>MGFLVMIREVSMAKAIRVVLLCVSVLWVVPKECACRSNFSRNSSSSSSSSLRPLRQRPSSVNVGALFTYDSFIGRAAKPAVKAAMDDVNADQSVLKGIKLNIIFQDSNCSGFIGTMGALQLMENKVVAAIGPQSSGIAHMISYVANELHVPLLSFGATDPTLSSLQFPYFLRTTQNDYFQMHAIADFLSYSGWRQVIAIFVDDECGRNGISVLGDVLAKKRSRISYKAAITPGADSSSIRDLLVSVNLMESRVFVVHVNPDSGLNVFSVAKSLGMMASGYVWIATDWLPTAMDSMEHVDSDTMDLLQGVVAFRHYTIESSVKRQFMARWKNLRPNDGFNSYAMYAYDSVWLVARALDVFFRENNNITFSNDPNLHKTNGSTIQLSALSVFNEGEKFMKIILGMNHTGVTGPIQFDSDRNRVNPAYEVLNLEGTAPRTVGYWSNHSGLSVVHPETLYSRPPNTSTANQRLKGIIYPGEVTKPPRGWVFPNNGKPLRIGVPNRVSYTDYVSKDKNPPGVRGYCIDVFEAAIELLPYPVPRTYILYGDGKRNPSYDNLVNEVVADNFDVAVGDITIVTNRTRYVDFTQPFIESGLVVVAPVKEAKSSPWSFLKPFTIEMWAVTGGFFLFVGAMVWILEHRFNQEFRGPPRRQLITIFWFSFSTMFFSHRENTVSSLGRFVLIIWLFVVLIINSSYTASLTSILTIRQLTSRIEGIDSLVTSNEPIGVQDGTFARNYLINELNILPSRIVPLKDEEQYLSALQRGPNAGGVAAIVDELPYIEVLLTNSNCKFRTVGQEFTRTGWGFAFQRDSPLAVDMSTAILQLSEEGELEKIHRKWLNYKHECSMQISNSEDSQLSLKS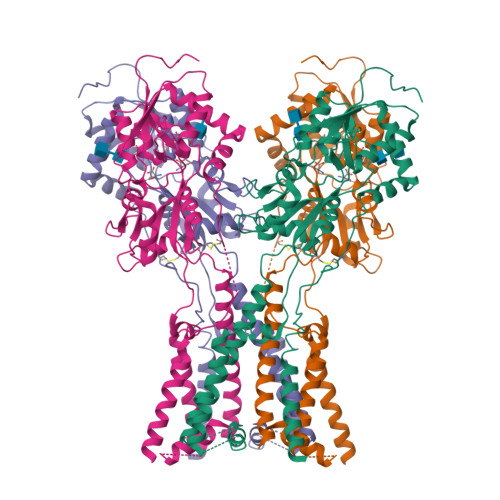FWGLFLICGITCFMALTVFFWRVFWQYQRLLPESADEERAGEVSEPSRSGRGSRAPSFKELIKVVDKREAEIKEILKQKSSKKLKSTQSAAGTSQSQHGEIT[4x]> MRGSHHHHHHGSADAYPSKAIRVIVPFAPGGSTDIIARLVTQRMSQELGQPMVVENKGGAGGAIGASEAARAEPDGYTLSIATVSTMAVNPACRPKDLPYDPIKDFQPVTNFANTANVVAVNPKFPAKDFKGFLEELKKNPGKYSYGSSGTCGVLHLMGESFKMATGTDIVHVPYKGSGPAVADAVGGQIELIFDNLPSSMPQIQAGKLRAMAIAWPTRIDAIKDVPTFADAGF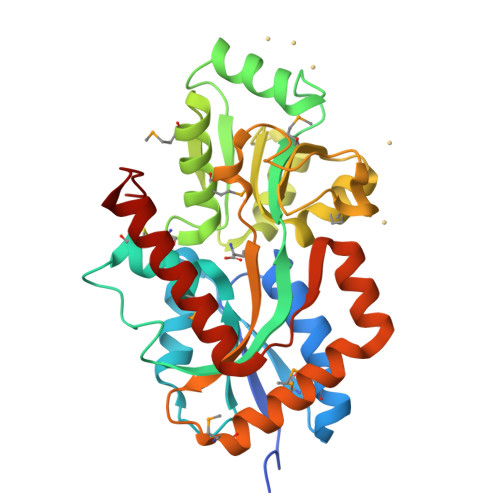PVLNQPVWYGLLAPKGTPMDVVNKLRDAAVVALKDPKVIKALDDQGSAPSGNTPEEFAKEIKEQYDWAQDVVKKQNIKLD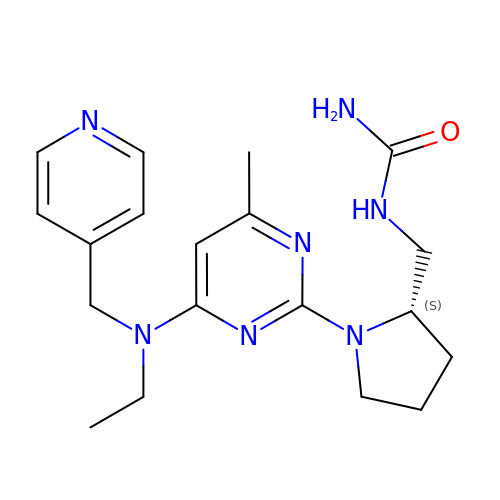1-[[(2~{S})-1-[4-[ethyl(pyridin-4-ylmethyl)amino]-6-methyl-pyrimidin-2-yl]pyrrolidin-2-yl]methyl]urea | C19 H27 N7 O | HHACEXLLNHJLFT-INIZCTEOSA-N>MELENYEQPVVLREDNRRRRRRMKPRSTAASLSSMELIPIEFVLPTSQRNTKTPETALLHVAGHGNVEQMKAQVWLRALETSVSADFYHRLGPDHFLLLYQKKGQWYEIYDKYQVVQTLDCLRYWKVLHRSPGQIHVVQRHAPSEETLAFQRQLNALIGYDVTDVSNVHDDELEFTRRRLVTPRMAEVAGRDPKLYAMHPWVTSKPLPEYLLKKITNNCVFIVIHRSTTSQTIKVSADDTPGTILQSFFTKMAKKKSLMDIPESQNERDFVLRVCGRDEYLVGETPIKNFQWVRQCLKNGEEIHLVLDTPPDPALDEVRKEEWPLVDDCTGVTGYHEQLTIHGKDHESVFTVSLWDCDRKFRVKIRGIDIPVLPRTADLTVFVEANIQYGQQVLCQRRTSPKPFTEEVLWNVWLEFSIKIKDLPKGALLNLQIYCGKAPALSGKTSAEMPSPESKGKAQLLYYVNLLLIDHRFLLRHGEYVLHMWQLSGKGEDQGSFNADKLTSRTNPDKENSMSISILLDNYCHPIALPKHRPTPDPEGDRVRAEMPNQLRKQLEAIIATDPLNPLTAEDKELLWHFRYESLKDPKAYPKLFSSVKWGQQEIVAKTYQLLAKREVWDQSALDVGLTMQLLDCNFSDENVRAIAVQKLESLEDDDVLHYLLQLVQAVKFEPYHDSALARFLLKRGLRNKRIGHFLFWFLRSEIAQSRHYQQRFAVILEAYLRGCGTAMLHDFTQQVQVIDMLQKVTIDIKSLSAEKYDVSSQVISQLKQKLENLQNLNLPQSFRVPYDPGLKAGALVIEKCKVMASKKKPLWLEFKCADPTALSNETIGIIFKHGDDLRQDMLILQILRIMESIWETESLDLCLLPYGCISTGDKIGMIEIVKDATTIAKIQQSTVGNTGAFKDEVLSHWLKEKCPIEEKFQAAVERFVYSCAGYCVATFVLGIGDRHNDNIMISETGNLFHIDFGHILGNYKSFLGINKERVPFVLTPDFLFVMGTSGKKTSLHFQKFQDVCVKAYLALRHHTNLLIILFSMMLMTGMPQLTSKEDIEYIRDALTVGKSEEDAKKYFLDQIEVCRDKGWTVQFNWFLHLVLGIKQGEKHSA[4x];>MESSDVELDFQRSVQAVLRELNTPNPALQSNQGMWRWSLHKKVERNPGKSSILVRILLRELEKAESEDGRRVIIPLLLTLMSVLTKATGIPEDL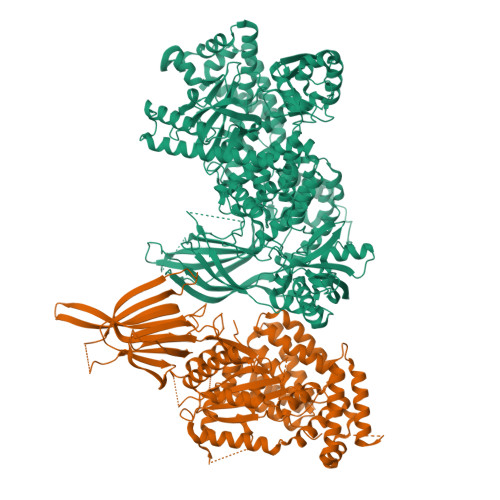YHRAYTFCTRLLTLPAPYSTVALDCAIRLKTETAVPGTLYQRTVIAEQNLISELYPYQERVFLFVDPELVSASVCSALLLEIQAAQEQQTPEACMRHVVSHALQAALGEACHTGALNRKLQASSRRVLEYYFHAVVAAIEQVASEDSPSRLGHLEKMEEIYCSLLGPATTRRHCVGDLLQDRLPSIPLPSPYITFHLWTDQEQLWKELVLFLRPRSQLRLSADLDALDLQGFRLDRDLARVSTDSGIERDLPLGSDELPDPSSSEMERAALQRKGGIKKRVWPPDFFMPGSWDGPPGLHRRTGRPSGDGELLPGVSRVHTARVLVLGDDRMLGRLAQAYYRLRKRETKKFCLTPRLSLQLYYIPVLAPQVTGQDPEASRKPELGELASFLGRVDPWYESTVNTLCPAILKLAEMPPYLDTSRTVDPFILDVITYYVRMGTQPIYFQLYKVKIFTSLSHDPTEDIFLTELKVKIQDSKSPKEGSSPRRRGAAEGTGAELSMCYQKALLSHRPREVTVSLRATGLVLKAIPAGDTEVSGFFHCTSPNAASATDCSCLHVSVTEVVKSSNLAGRSFTTSTNTFRTSSIQVQSQDQRLLTLWLDKDGRRTFRDVVRFEVSPCPEPCSRTQKSKTSALNSHGQETEKNMAKPNSLLMPINTFSGIIQ[4x]>STHFDVIVVGAGSMGMAAGYQLAKQGVKTLLVDAFDPPHTNGSHHGDTRIIRHAYGEGREYVPLALRSQELWYELEKETHHKIFTKTGVLVFGPKGESAFVAETMEAAKEHSLTVDLLEGDEINKRWPGITVPENYNAIFEPNSGVLFSENCIRAYRELAEARGAKVLTHTRVEDFDISPDSVKIETANGSYTADKLIVSMGAWNSKLLSKLNLDIPLQPYRQVVGFFESDESKYSNDIDFPGFMVEVPNGIYYGFPSFGGCGLRLGYHTFGQKIDPDTINREFGVYPEDESNLRAFLEEYMPGANGELKRGAVCMYTKTLDEHFIIDLHPEHSNVVIAAGFSGHGFKFSSGVGEVLSQLALTGKTEHDI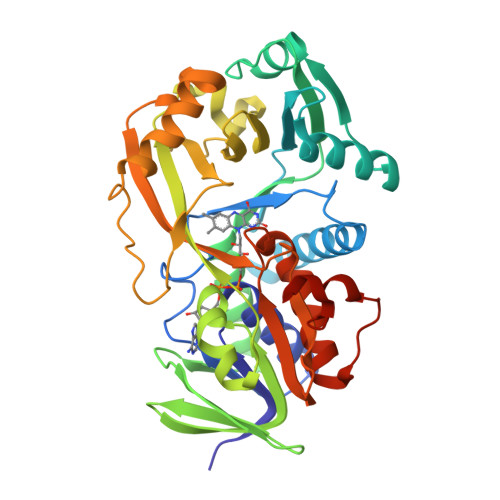SIFSINRPALKESLQKTTI[4x]>[2x]MIYEGKAITVTALESGIVELKFDLKGESVNKFNRLTLNELRQAVDAIKADASVKGVIVSSGKDVFIVGADITEFVENFKLPDAELIAGNLEANKIFSDFEDLNVPTVAAINGIALGGGLEMCLAADFRVMADSAKIGLPEVKLGIYPGFGGTVRLPRLIGVDNAVEWIASGKENRAEDALKVSAVDAVVTADKLGAAALDLIKRAISGELDYKAKRQPKLEKLKLNAIEQMMAFETAKGFVAGQAGPNYPAPVEAIKTIQKAANFGRDKALEVEAAGFAKLAKTSASNCLIGLFLNDQELKKKAKVYDKIAKDVKQAAVLGAGIMGGGIAYQSASKGTPILMKDINEHGIEQGLAEAAKLLVGRVDKGRMTPAKMAEVLNGIRPTLSYGDFGNVDLVVEAVVENPKVKQAVLAEVENHVREDAILASNTSTISISLLAKALKRPENFVGMHFFNPVHMMPLVEVIRGEKSSDLAVATTVAYAKKMGKNPIVVNDCPGFLVNRVLFPYFGGFAKLVSAGVDFVRIDKVMEKFGWPMGPAYLMDVVGIDTGHHGRDVMAEGFPDRMKDDRRSAIDALYEAKRLGQKNGKGFYAYEADKKGKQK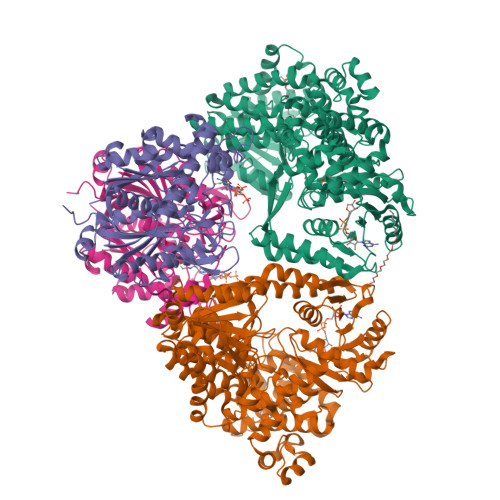KLVDSSVLEVLKPIVYEQRDVTDEDIINWMMIPLCLETVRCLEDGIVETAAEADMGLVYGIGFPLFRGGALRYIDSIGVAEFVALADQYAELGALYHPTAKLREMAKNGQSFFG;>[2x]SLNPRDVVIVDFGRTPMGRSKGGMHRNTRAEDMSAHLISKVLERNSKVDPGEVEDVIWGCVNQTLEQGWNIARMASLMTQIPHTSAAQTVSRLCGSSMSALHTAAQAIMTGNGDVFVVGGVEHMGHVSMMHGVDPNPHMSLYAAKASGMMGLTAEMLGKMHGISREQQDAFAVRSHQLAHKATVEGKFKDEIIPMQGYDENGFLKIFDYDETIRPDTTLESLAALKPAFNPKGGTVTAGTSSQITDGASCMIVMSAQRAKDLGLEPLAVIRSMAVAGVDPAIMGYGPVPATQKALKRAGLNMADIDFIELNEAFAAQALPVLKDLKVLDKMNEKVNLHGGAIALGHPFGCSGARISGTLLNVMKQNGGTFGLSTMCIGLGQGIATVFERV> MDPSSKPLREIPGSYGIPFFQPIKDRLEYFYGTGGRDEYFRSRMQKYQSTVFRANMPPGPFVSSNPKVIVLLDAKSFPILFDVSKVEKKDLFTGTYMPSTKLTGGYRVLSYLDPSEPRHAQLKNLLFFMLKNSSNRVIPQFETTYTELFEGLEAELAKNGKAAFNDVGEQAAFRFLGRAYFNSNPEETKLGTSAPTLISSWVLFNLAPTLDLGLPWFLQEPLLHTFRLPAFLIKSTYNKLYDYFQSVATPVMEQAEKLGVPKDEAVHNILFAVCFNTFGGVKILFPNTLKWIGLAGENLHTQLAEEIRGAIKSYGDGNVTLEAIEQM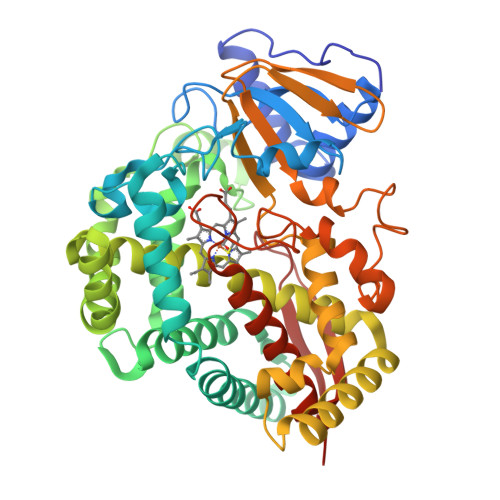PLTKSVVYESLRIEPPVPPQYGKAKSNFTIESHDATFEVKKGEMLFGYQPFATKDPKVFDRPEEYVPDRFVGDGEALLKYVWWSNGPETESPTVENKQCAGKDFVVLITRLFVIELFRRYDSFEIELGESPLGAAVTLTFLKRASI>DSELQLVEQRIRSFPDFPTPGVVFRDISPVLKDPASFRAAIGLLARHLKATHGGRIDYIAGLDSRGFLFGPSLAQELGLGCVLIRKRGKLPGPTLWASYSLEYGKAELEIQKDALEPGQRVVVVDDLLATGGTMNAAC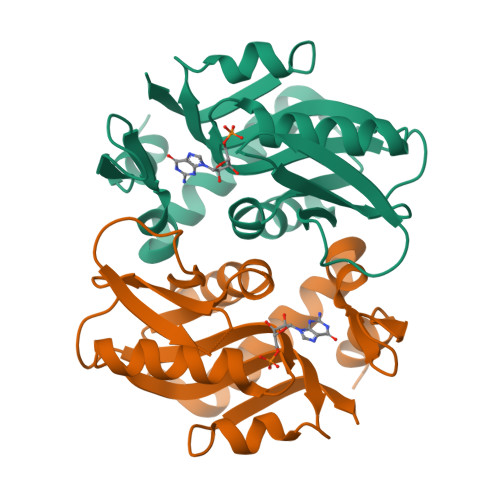ELLGRLQAEVLECVSLVELTSLKGREKLAPVPFFSLLQYE[2x]(3S,3aR,6S)-3,7,7,8-tetramethyl-2,3,4,5,6,7-hexahydro-1H-3a,6-methanoazulene | C15 H24 | 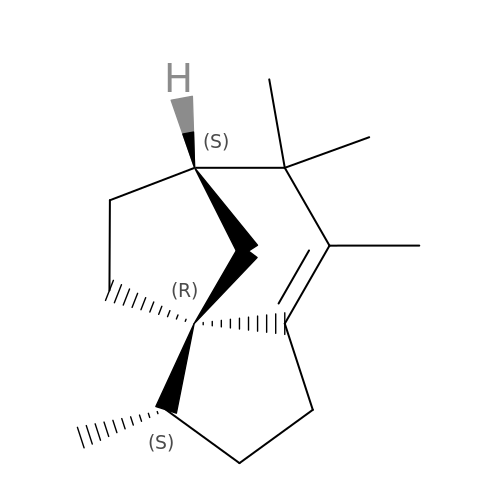CYLSPJUZBPWJGC-ITDIGPHOSA-N The selective autophagy receptor p62/SQSTM1 is known to form higher-order filaments in vitro and to undergo liquid-liquid phase separation when mixed with poly-ubiquitin. p62 has a key role in selective autophagy by recognizing poly-ubiquitinated cargo and delivering it to the autophagosome. At the early stages of autophagy, selective autophagy receptors like p62 thereby bridge ubiquitinated cargo via conjugated Atg8 to the forming autophagosome.

In order to improve our detailed structural understanding of purified p62, we determined the cryo-electron microscopy (cryo-EM) structure of full-length p62. Therefore, we recorded a full cryo-EM data set at pH 6.0 revealing long and flexible filaments with a width of approximately 15 nm. Due to pitch heterogeneity between 130 and 160 Å, we refined a more homogeneous subset with a 150 Å pitch and 13.6 units per turn (corresponding to 11.0 Å helical rise and a −26.1° helical rotation), including dihedral symmetry and obtained a 3D reconstruction at 4.5 Å global resolution. Consistent with the class averages, the local resolution varied significantly from a well-defined PB1 domain scaffold at 4.2 Å resolution up to over 9 Å for the more flexible regions. The cryo-EM structure revealed a left-handed double-helical filament with two antiparallel strands of PB1 domains in the full-length p62 assembly. At lower density thresholds, the ZZ domain envelope emerged connected to the PB1 domain, albeit at lower resolution. The densities of the associated C-terminal domains were weak and poorly resolved as they did not follow helical symmetry, presumably due to molecular flexibility with respect to the PB1 strands, which is in agreement with the assigned structurally disordered region in residues 169–33821. In comparison, the here determined full-length structure revealed only two well-resolved antiparallel PB1 scaffold strands, resulting in an open major groove, while the previously determined PB1 domain-only assemblies had one or two additional PB1 strands inserted into the closed helical assembly. In the full-length structure, the space required by the additional 340 C-terminal amino acids restricts the assembly to two antiparallel PB1 strands, leaving space for a major groove. In contrast, our full-length p62 filament structure was solved at pH 6 in order to obtain a more homogeneous closed filament conformation following the helical symmetry.

>[40x]ASLTVKAYLLGKEDAAREIRRFSFCCSPEPEAEAEAAAGPGPCERLLSRVAALFPALRPGGFQAHYRDEDGDLVAFSSDEELTMAMSYVKDDIFRIYIKEKKEC>[2x]MRVLLIHSDYIEYEVKDKALKNPEPISEDMKRGRMEEVLVAFISVEKVDEK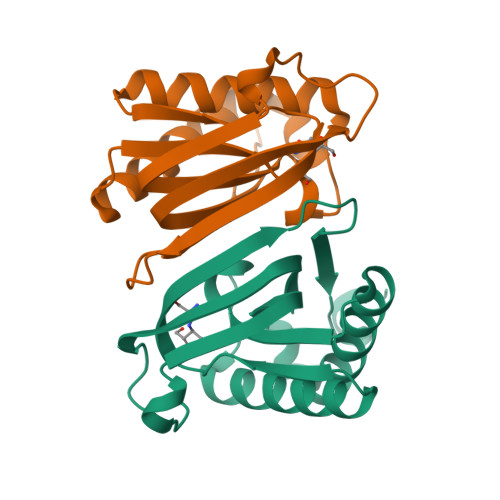NPEEVSLKAIEEISKVAEQVKAENVFVYPFAHLSSELAKPSVAMDILNRVYQGLKERGFNVGKAPFGYYKAFKISCKGHPLAELSRTIVPEEARVE>[2x]NNNG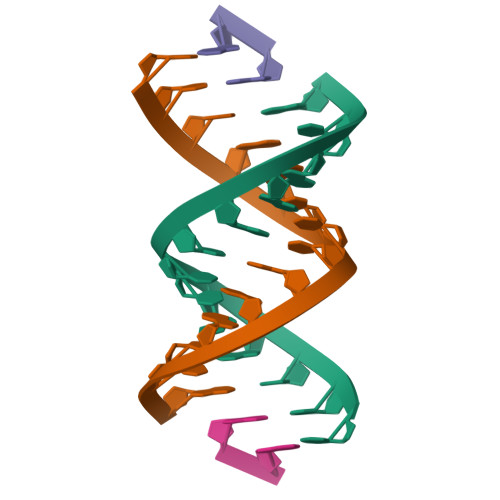ACUUAAGUCG;>GG[2x]1-methyl-3-oxidanyl-pyridine-2-thione | C6 H7 N O S | 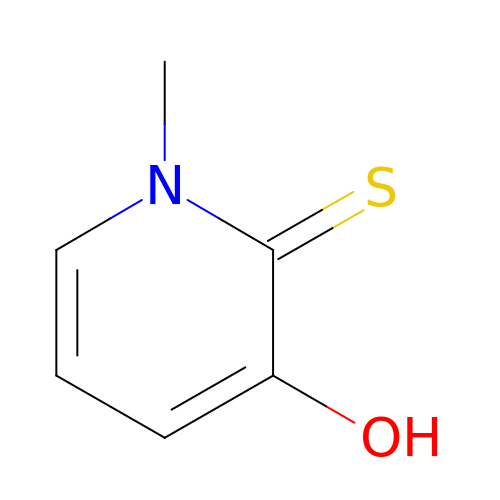SQEXIHSVVCJZTQ-UHFFFAOYSA-N In mitosis, the augmin complex binds to spindle microtubules to recruit the γ-tubulin ring complex (γ-TuRC), the principal microtubule nucleator, for the formation of branched microtubules. The elongated structure of the augmin complex is characterised by extensive coiled-coil segments and comprises two structural elements with distinct but complementary functions in γ-TuRC and microtubule binding, linked by a flexible hinge. The augmin complex is recruited to microtubules via a composite microtubule binding site comprising a positively charged unordered extension and two calponin homology domains. By acting as an elongated structural scaffold, augmin positions the γ-TuRC on the pre-existing microtubule in a partially flexible manner, allowing the γ-TuRC to nucleate a branched microtubule in an approximate orientation with respect to the mother microtubule.

Since expression of the isolated TII tetramer is reportedly inefficient and structural characterisation by negative stain EM analysis failed, we opted for co-expression of all eight augmin subunits to reconstitute the augmin holocomplex. We subjected the negatively stained augmin particles to 3D classification to obtain a 3D reconstruction of the augmin holocomplex in a defined conformational state, in which the TIII tetramer could be unambiguously identified. The remaining density clearly reflected the clamp-like overall shape of the predicted TII tetramer models and the hammerhead-like region formed by the N-termini of TII HAUS proteins was recapitulated in the density, allowing us to confidently determine the orientation of TII in the 3D reconstruction. The approximate placement of the predicted TII tetramer into the negative stain 3D class indicated an interaction between the TIII H3/H5-arm and the TII C-clamp. Guided by these insights into the overall organisation of the augmin holocomplex, we used AlphaFold-Multimer to predict the structure of the TIII H3/H5-arm in combination with the TII tetramer. In all predicted models, the TII C-clamp interacts with the periphery of the TIII H3/H5-arm in a manner that is fully compatible with the negative stain 3D reconstruction of the augmin holocomplex, as judged by seamless fit of the composite TIII tetramer-TII C-clamp model into the EM density, thus providing an accurate model for the interface between the TII and TIII tetramers. We thus individually docked the TII N-clamp as a rigid body into the remaining density segments guided by the orientation of the N-clamp HH. Merging the TII N-clamp with the model for the TII C-clamp in complex with TIII, we generated a model for the complete augmin holocomplex. The N-clamp is linked to the TII C-clamp by a hinge region, which allows for an opening and closing motion of the TII clamp, as suggested by the ensemble of predicted models.

> MDEKSTKIIMWLKKMFGDKPLPPYEVNTRTMEILYQLAEWNEARDKDLSLVTEDLKLKSAEVKAEAKYLQDLLTEGLGPSYTNLSRMGNNYLNQIVDSCLALELKNSSLSSYIPAVNDLSSELVAIELNNQEMEAELTSLRKKLTEALVLEKSLERDLKKAEEQCNFEKAKVEIRSQNMKKLKDKSEEYKYKIHAAKDQLSSAGMEEPLTHRSLVSLSETLTELKAQSMAAKEKLNSYLDLAPNPSLVKVKIEEAKRELKATEVELTTKVNMMEFVVPEPSKRRLK;> MSGGDRFVQTLQKLNYPKGAQLDGEDFDWLFEAVDLKPFLDWFCSAASEQNVVPDEKLQAFNTLKESGKPVLDEKALDEVLKTFSISKVPAIEEVAIEKLEEEVKALQKQKNLHIRRRNKLQMVESGNRQMCLKSKDKEEETGRAFQEVLHLLRVTNKKLNHELQSIVNGVQTLMSFFSTPETACELSSQPIFLSQLLLDKYLSLEEQSTAALTSFTKEHFFEGMSKFVEGSDENFQLVQLNVNSFGEDGTTEDKCKEMMRLQLAYICAKHKLIQMKAKSASLKVGLQWAENNASVVQDKASQKEENLKVRITSLKNETLQIENHTNSISNEKLPGLVRDNAQLLNMPIVKGDYDLQMAHQTSCSSRQDLVCDHLMKQKASFELLQLGYELELRKHRDVYRELGSIVQELKESGDKLEERLTMLSDVNLLSASKPRSNIDSKDLTSHRLYQLLDGDNTQKLFRTYDGLESVAQKLSQDIASMRDQLEVSEQEHSLLLSKLDSHLKELRDFMYPEGNTLMLTTPELSGEFHQLGSQLEKLNHITVEILGDLQLKRKMLESNKLQQIEKQLYVYFFQNEEQLKSIVGKLEAQTGGGSSA;> MAQTLQYVSSRLSMLQIDEEDLERNAQFGKVLIELCPLLGPNGGSANLNRELEETRRELLLQRKMWMRSEVIYQLVQEMLLDLQVRKLEGSLTEEERKFQDGLQQCMLVSECSRLLTADSVPPSDSTSILGLDKQDLLDLLPPNMLVLWVRDRLQKQLEEALKKKCFTFLSFHQPETDEEGDVLRAAKVLRLASTLEDEKRRLQNEQEKHQEMRALLEKQQEIYPHVLLRCLSLLRQAASELRLRAQSDIDRINAEYLEAKSNALFLKLRMEELQVLTDCYTPEKVLVHRQIRDTLEAGVKKEKQELSTSRQILSSYEFLGPEFEGLVQEYTRLKDKIKDNRWMLQELSKSLP;> MERRSLAQELKKWAVEEMGLPAQKAPSEEMLQRLFIGQCGDIWKFIIRHIHSHRTVRKIEGNLLWYQQLQHTEAQRTAEEEQQQRRKQLCKEILELRAELHHLQEQIQTAEREIVGQDLNCERAQDLCRRSLLLRAFNKKREEECEALCQSNKKIQYRCEQLQEIRRASQREVMFSAVDPDLSSSTFLEPEVLRDVREVCKLRFKFLRSLHDDSISSSVHPGKEDLRSLSHQQWMSMAEKVWNTHTPNHILAALERLTLNSTQELKKLQFSQAADLSKGPSCQLKEFSEPITQSRSCNESTHLDPQETLPSFHSLIQEGWANSVKVSSELRRVQSQAQALSEHLAERIQEIHKKLSDGSEVSVLTRAAFDAELRCVILRGCRDALMQECRMLQEEAAGKKQEMKLLQQQQQNIQEACLLLDKKQKHIQILIKGNSSSKSQIRRSSVEAQKYVQDKLLPWPQEIIQESQRLQDSIQKEVKHFSAICLPALLKVSTDGFNLLPSRELSINRMSNTHAPYYGIFKGIYESVRLPLYKAPESVLSHVADMKKQLFFLRSQLSSRSEAISKTQRALQKNTNPDTDALLKSLSDHYSLELDEMVPKMQRLIQQCEKHQEYGKEVQATVMDWWEQPVQLCLPSEERGGLTLRQWRERWTVAVTALQRATGSRS;> MMAANPWSPVQPSAASLLLEKCLAAGVLSQNALDQAQLEAPCFSHAEELQRITEIKAEINQKSLELELLRLEKETADITHPLYLGQKHQALQAMNSHLEAVLREKRSLRQRLAQPVCQENLPIEASYHRFTAELLPLAVNFIEKLEIYIKTIQTIPKIPDCASNMDNALMRMESLEAEMEEVTEQILTWREQQKTAFQMNSDANSSCITAQTSYLSIENLHP;> MQSGSRPHLAWQREHMWLALQGLGFESGAEAANAGKTLVHVTFGVNMFDKPNKDAFYVVFHFLFGKLDNVRCKEVFRYCWPPLDKKRDAEFRKACCEWLKKISDEVGAGFPQVVASIFLSPGGPKFVHLLYHFARYVMLQHIKRDADAGNVFISEALQSKIQDPQKALARNKLARQKYLKVLQKENLVIEEYQRKAQLLIKQIRDMRSEHVALQNQQKLAEKVDRKISDKDENIQKTRCMWNTIMQMLKEMEKEVDVVDAVVRGNIDQYCLDGTNATLNIPNLLISRIESEMHRLQMDNVYEAGKVNLITVVQLLNEALKLVSGERSLYDCKGVRLDLQYLHGKAKFESEVLTRLRNMRHKIKREDLVSIEKIIADREREWERKWEKILGKCPFSLLKGLNPALELNPPMAPFSFDPASEEVLKSSVFCHYPASLQEYSHKEKPLKDFNQDHSGELVQRLIGATVLTRSGRKSTSSLGMATPNRRRMSLNEREFQTPTMNDRIGFQRTPSSAVQKRRADVSWKTAANSPLPCTPTPYKQDPKNMARQQLAQQVADYIVSESPRSSGGRGMELDDLLGVLSSDPFLSRKEIPRTPENLISDIRSSWRKAIQSEESLVVASPVAAPCMDSTAELESAHCSQIDLSMACFLSTSHASDQNDCSGTRIPHNTGGNKASSLHSDVVHHESIDMKSEIDSSQPEDLSLPIKENEPADKLINLLDDKKESENADTLTNPVEFIFSNQPISKLMDKTMFISVSGQENLSAHTTLSWNSSNMITSDSSSDTHEIIQFGILHETLPENAGNVSLNSTLSLGGNEEPFEKSELSDHDFTFDRKEHSSRSMEGKMDINSIRSRYEALKRTLTSLTDEEYHGDPDTSNMRFTKHKSESSLILGSDVYSPVEKVLSLDLEYLTTPSPKDRKLSLPQLISFSPETIRSEKQEDLLDVFESQDFVNPNKTFDFTSSGLDLQKSTDEGPEQLIKL;> MTGGKELGAAVELYERLQMLSCPCLEGVYLTDPQSIYELLCTPSSHRLDILQWLCSRIYPPVQEQLSSLKESQTDTKVKEIAKLCFDLMLCHFDDLDLIRGHASPFKQISFIGQLLDVIQYPDTISSNVILESLSHSTEKNVVTCIRENEELLKELFSSPHFQATLSPECNPWPADFKPLLNAEESLQKRATQSSKGKDMSNSVEALLEISSSLKALKEECVDLCSSVTDGDKVIQSLRLALTDFHQLTIAFNQIYANEFQEHCGHPAPHMSPMGPFFQFVHQSLSTCFKELESIAQFTETSENIVDVVRERHQSKEKWAGSTISTLCEKMKELRQSYEAFQQSSLQD;> MSEAGVAPIEDGSQNSSGGSSGDAALKKSKGGAKVVKSRYMQIGRSKVSKNSLANTTVCSGGKVPERGSGGTPTRRSLAPHKAKITAAVPLPALDGSIFTKEDLQSTLLDGHRIARPDLDLSVINDRTLQKITPRPVVTSEQKKPKRDTTPVNLVPEDMVEMIESQTLLLTYLTIKMQKNLFRLEEKAERNLLLVNDQKDQLQETIHMMKRDLTLLQREERLRDLIEKQDEVLTPVVTSKDPFKDNYTTFATALDSTRHQLAIKNIHITGNRHRYLEELQKHLAITKSLLEEIMPSHASENAESFDTIKDLENIVLKTDEELARSFRQILDLSFKVNKEISLQSQKAVEETCESALVRQWYFDGSLP>[4x]MRGSHHHHHHGSLSSSPSEILQELGKGSTHPQPGVSPPAAPAAPGPKDGPGETDAFGNSEGKELVASGENKIKQGLLPSLEDLLFYTIAEGQEKIPVHKFITALKSTGLRTSDPRLKECMDMLRLTLQTTSDGVMLDKDLFKKCVQSNIVLLTQAFRRKFVIPDFMSFTSHIDELYESAKKQSGGKVADYIPQLAKFSPDLWGVSVCTVDGQRHSTGDTKVPFCLQSCVKPLKYAIAVNDLGTEYVHRYVGKEPSGLRFNKLFLNEDDKPHNPMVNAGAIVVTSLIKQGVNNAEKFDYVMQFLNKMAGNEYVGFSNATFQSERESGDRNFAIGYYLKEKKCFPEGTDMVGILDFYFQLCSIEVTCESASVMAATLANGGFCPITGERVLSPEAVRNTLSLMHSCGMYDFSGQFAFHVGLPAKSGVAGGILLVVPNVMGMMCWSPPLDKMGNSVKGIHFCHDLVSLCNFHNYDNLRHFAKKLDPRREGGDQRHSFGPLDYESLQQELALKETVWKKVSPESNEDISTTVVYRMESLGEKS

Cancer cells often overexpress glutaminase enzymes, in particular glutaminase C (GAC), which resides in the mitochondria and catalyzes the hydrolysis of glutamine to glutamate. Glutamate is then either used to fuel the TCA cycle via its conversion to α-ketoglutarate by glutamate dehydrogenase or as a building block for various biomolecules. Numerous GAC inhibitors have been reported, with the most heavily investigated being a class of compounds derived from the small molecule bis-2-(5-phenylacetamido-1,3,4-thiadiazol-2-yl)ethyl sulfide (BPTES). These compounds bind at the dimer/dimer interface of the GAC tetramer, which is near the so-called activation loop (Gly315 to Glu325), effectively trapping the tetrameric enzyme in an inactive conformation.

The serial room temperature crystal structure that was solved for the GAC-UPGL00004 complex was largely similar to the corresponding high-pressure cryo-cooled structure, with the two inhibitor molecules bound to the GAC tetramer exhibiting the same cup-shaped orientation routinely observed in the cryo-cooled structure for this complex. By contrast, both molecules of UPGL00004 bound to GAC in the room temperature X-ray structures adopted the more typical cup-shaped orientation within the binding site. This supports the idea that UPGL00004 is held rigidly in the allosteric binding site of GAC, whereas BPTES, even when bound to the enzyme, has a significant degree of conformational flexibility. In this case, the ring-to-ring distance is 18.5 Å, which is significantly larger than the distances between the rings in either the cryo-cooled structure (14.4 Å) or for the UPGL0004 molecule (14.6 Å in the cryo-cooled structure and 14.7 Å in the room-temperature structure).>[2x]VMKQYLSRLASLTLFVGFMSAAQAAVAPLDLVQPISDYKIYVSENLQTLVRDTR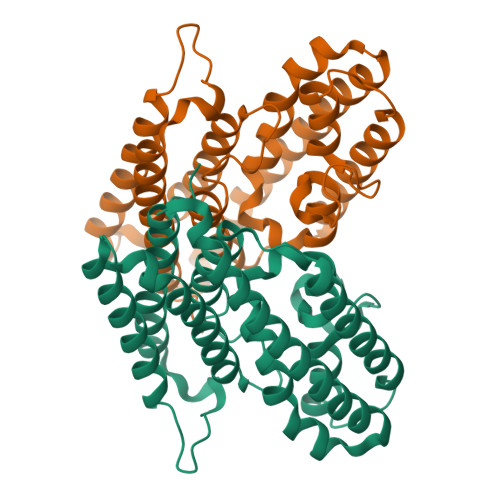EFTNAVKAGDVAKAKKLFASTRMSYERIEPIAELFSDLDASIDSRADDHEKAEKDPAFFGFHRIEYGLFAQNSAKGLAPVADKLMADVLELQKRIRGLTFPPEKVVGGAAVLMEEVAATKISGEEDRYSHTDLWDFQANFEGAKKIVDLFRPLVVKDNRAFADKVDANFDTVFKTLAKYRTADGGFELYGKLSERDRKVLAGRVNTLAEDLSKMRGLLGLDLEHHHHHH>[2x]GFGELKEEWRGEVVHLSWSPRAFLLKNFLSDEECDYIVEKARPKMVKSSVVDNESGKSVDSEIRTSTGTWFAKGEDSVISKIEKRVAQVTMIPLENHEGLQVLHYHDGQKYEPHYDYFH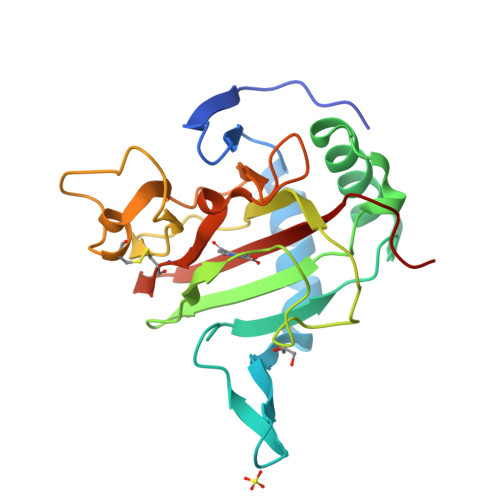DPVNAGPEHGGQRVVTMLMYLTTVEEGGETVLPNAEQKVTGDGWSECAKRGLAVKPIKGDALMFYSLKPDGSNDPASLHGSCPTLKGDKWSATKWIHVAPIGGRH> APGQKECDNALRQLETVRELLENPVQPINDMSYFGCLDSVMENSKVLGEAMTGISQNAKNGNLPEFGDAIATASKALCGFTEAAAQAAYLVGVSDPNSQAGQQGLV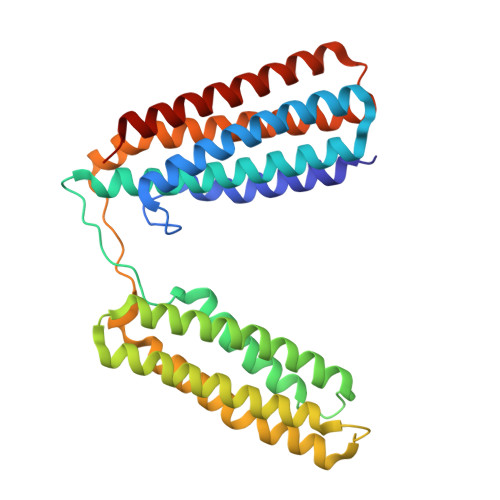EPTQFARANQAIQMACQSLGEPGCTQAQVLSAATIVAKHTSALCNSCRLASARTANPTAKRQFVQSAKEVANSTANLVKTIKALDGDFTEENRAQCRAATAPLLEAVDNLSAFASNPEFSSVPAQISPEGRAAMEPIVISAKTMLESAGGLIQTARALAVNPRDPPRWSVLAGHSRTVSDSIKKLITSMRDKAPG> KFE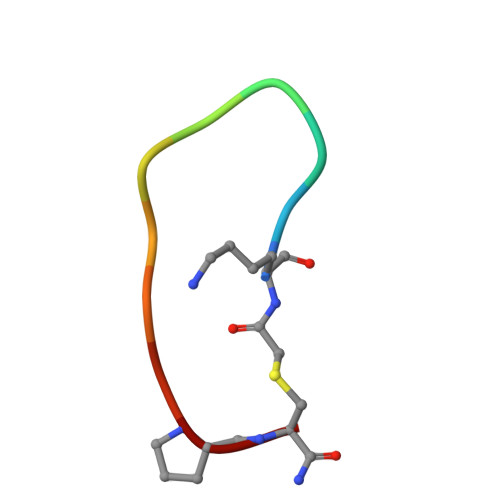GYDNEFPX>[2x]SVKLAGNSSLCPVSGWAIYSKDNSVRIGSKGDVFVIREPFISCS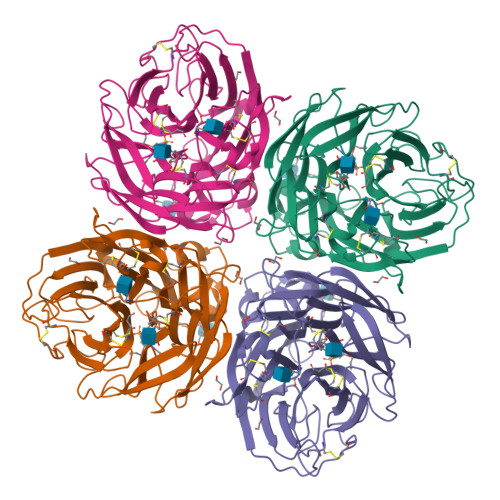PLECRTFFLTQGALLNDKHSNGTIKDRSPYRTLMSCPIGEVPSPYNSRFESVAWSASACHDGINWLTIGISGPDNGAVAVLKYNGIITDTIKSWRNNILRTQESECACVNGSCFTVMTDGPSNGQASYKIFRIEKGKIVKSVEMNAPNYHYEECSCYPDSSEITCVCRDNWHGSNRPWVSFNQNLEYQIGYICSGIFGDNPRPNDKTGSCGPVSSNGANGVKGFSFKYGNGVWIGRTKSISSRNGFEMIWDPNGWTGTDNNFSIKQDIVGINEWSGYSGSFVQHPELTGLDCIRPCFWVELIRGRPKENTIWTSGSSISFCGVNSDTVGWSWPDGAELPFTID> MFLKRLDVIGFKSFAERISVDFVKGVTAVVGPNGSGKSNITDAIRWVLGEQSARSLRGGKMEDIIFAGSDSRKRLNLAEVTLTLDNDDHFLPIDFHEVSVTRRVYRSGESEFLINNQPCRLKDIIDLFMDSGLGKEAFSIISQGKVEEILSSKAEDRRSIFEEAAGVLKYKTRKKKAENKLFETQDNLNRVEDILHELEGQVEPLKIQASIAKDYLEKKSGGSLIKLAIEELG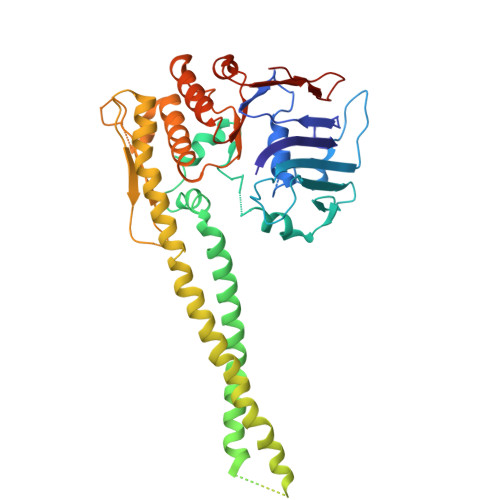TVNLGSIDEFERVNERYKFLSEQKEDLTEAKNTLFQVIEEMDEEMTKRFNDTFVQIRSHFDQVFRSLFGGGRAELRLTDPNDLLHSGVEIIAQPPGKKLQNLNLLSGGERALTAIALLFSILKVRPVPFCVLDQVEAALDEANVFRFAQYLKKYSSDTQFIVITHRKGTMEEADVLYGVTMQESGVSKVISVKLEETKEFVQ> MGHHHHHHMMTVGLYLYGIFPEPIPDGLVLQGIDNEPVHSEMIDGFSFLYSAAHKEKYLASRRYLICHEKVLETVMEAGFTTLLPLRFGLVIKTWESVTEQLITPYKTQLKELFAKLSGQREVSIKIFWDNQWELQAALESNPKLKQERDAMMGKNLNMEEIIHIGQLIEATVLRRKQDIIQVFRDQLNHRAQEVIESDP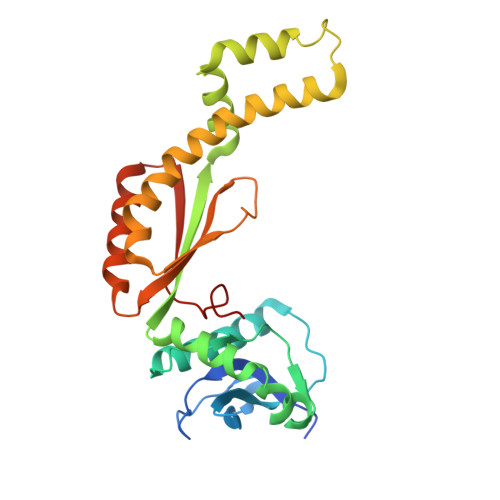MTDDMIYNAAYLIPWEQEPEFSQNVEAIDQQFGDRLRIRYNNLTAPYTFAQLI1,2,4-TRIAZOLE-CARBOXAMIDINE 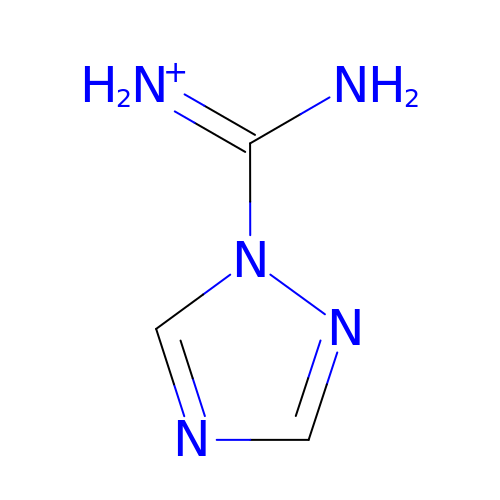| C3 H6 N5 | CDIOIIJXUJXYPB-UHFFFAOYSA-O>MTGPEPVPAGPPPDPTPPRRAGSVWAHVGQHFTEEAFDIVVIGAGRMGAACAFYLRQLAPGRSLLLVEEGGLPNEEGATILAPGVWTAQDIPAGQEAQAEWTREQLLGALGSGKTLEVEDRPLLHLLPAGEGSGLTPTLDALADFPEALALLDPARLPVARVDPRALTYRPGSLALLAAQQAIGQGAGLLLNTRAELVPGGVRLHRLTVTNTHQIVVHETRQIRAGVIIVAAGAAGPALV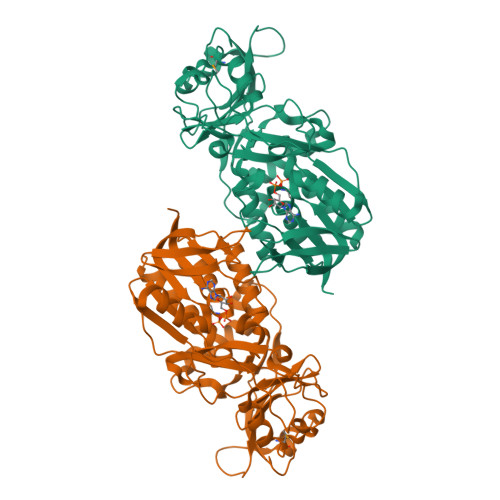EQGLGLHTRHGRAYRQFPRLDLLSGAQTPVLRASGLTLRPQNGGYTLVPAIHHRDPHGYHPAGGSLTGVPTGLRRELLEDLVGLMDAVPALAGEGLELGRSSADVPGAWLALPGGRPDAPPQAEELAPGLHLLLGGPLADTLGLAAAHELAQRVSASLEHHHHHH[2x]>[2x]GPLGSFGQTTPPLVDFLKDILRRYPEGGQILKELIQNAEDAGATEVRFLYDETQYGNESLWSKDMAQYQGSALYVYNNAIFTPEDWHGIQEIARSRKKDDPLKVGRFGIGFNSVYHITD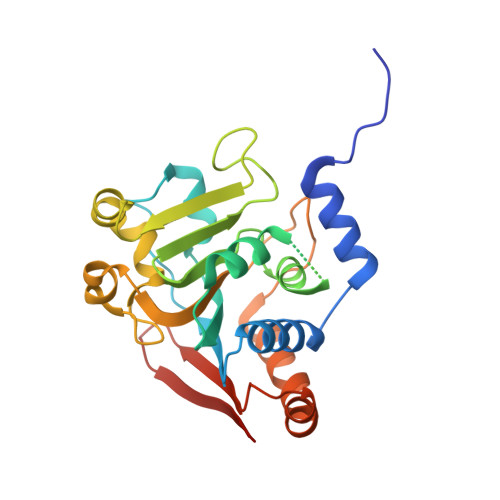VPSIFSGDQIGMLDPHQTLFGPHESGQCWNLKDDFKEMNELTDQFAPFIGVFGSTKETFQNGHFPGTFFRFPLREQPSQLSSNIYNKEKVLELFDSFRADADTVLLFLKSVQDVSLHVREADGTERLIFRVTAS> SAKEKFTSLSPAEFFKRNPELAGFPNPARALYQTVRELIENSLDATDVHGILPNIKITIDLIDDARQIYKVNVVDNGIGIPPQEVPNAFGRVLYSSKYVNRQTRGMYGLGVKAAVLYSQMHQDKPIEIETSPVNSKRIYTFKLKIDINKNEPIIVERGSVENTRGFHGTSVAISIPGDWPKAKSRIYEYIKRTYIITPYAEFIFKDPEGNVTYYPRLTNKIPKPPQEVKPHPYGVDREEIKILINNLKRDYTIKEFLVNEFQSIGDTTADKILELAGLKPNKKVKNLTEEEITRLVETFKKYEDFRSPSADSLSVIGEDL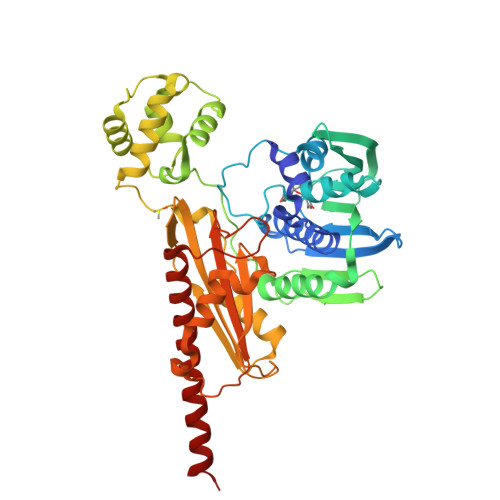IELGLKKIFNPDFAASITRKPKAYQGHPFIVEAGVAFGGSIPVGEEPIVLRYANKIPLIYDEKSDVIWKVVEELDWKRYGIESDQYQMVVMVHLCSTKIPYKSAGKESIAEVEDIEKEIKNALMEVARKLKQYLSEKRKEQEAKKKLLA> MTPHLMKLL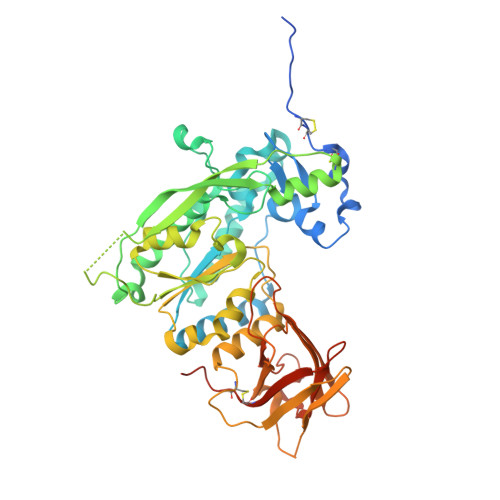GLSAALLAISQGVRAEDVKAPTFSAEPCCQLCPEAHDASRYTTRYQQNFTTLVQAQGDWLFRTREDLRTEFNTTPAGYKRLQQVHDAFKKRGVELVVVYQPTRGLVNRNMLNPAEKAAFDYQKALGNYQAMLKRFASMGYNVPDLSPLTNEQLAAADQGKDFYFRGDQHWTPYGAERAAKIVADTVHKMPAFEGIPRKEFETRKSGRMGKTGTLHNVAGQLCGTSYAVQYMDQFATEPKGASGGDDLFGDSGNAQITLVGTSHSGKNYNFSGFLEQYIGADVLNVAFPGGGLEGSMIQYLGSEEFQKNPPKILIWEFSPLYRLDQETIWRQILGLLDDGCDDRPALMSASTTLKPGKNELMVNGKGGVIKDLINRNLQMDVKFEDPSVKVLQATLWYLNGRHEDIKLEKPETSDTDGRFVFQMREDEDWASQRLLAFEVQGPESGTQKVEAKLCKRNNFAVPAQTAQAGQLEHHHHHH> UCCGUGAUAGUUUAAUGGUCAGAAUGCCAGACUGAAGAUCUGGAGAUCGGGGUUCAAUUCCCCGUCGCGGAGCC;> UUU;> GCGGAUUUAGCUCAGUUGGGAGAGCGCCCGCUUGUCGCGUGGGAGGUCCUGUGUUCGAUCCACAGAAUUCGC;> GUC;> UCCGU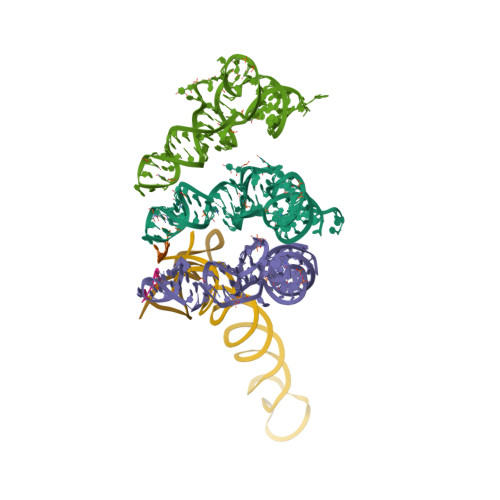GAUAGUUUAAUGGUCAGAAUGGGCGCUUGUCGCGUGCCAGAUCGGGGUUCAAUUCCCCGUCGCGGAG;> CGUCACACCAUGGAAGGGGGUUGCAAAGAAAGGGUGGCCCCCUUCGGGGCGCCUAACUUUGUGAUUCCUAACUGGGGUGAAGUCG;> CUGGGGAGUACGGCCGCAAGGCUGAAACUCAAA> MNNKLMNIIELIRKDTGINNAIDAVEQLALLLLVRYTHEVASNEISKENHIDSFKNLFFDLNDFSKDGLVIDFYTLRDKLNHIVVNCRFSENELSHSVFSRNNWEKIENILDQIPFRIRSTKILDLVIHRLEELDLSEGIEIDFDHLLLNMVKDSGSSGAYYSPRPLIKAMVRVLNPKPLATVYDPAMGTGGVFVEAKKHAKGKSCFNGLSFIGNDLSPFAHLIGALNLLLNDIDISGVSISDSLLDRDCQQYDFVISGVPFGKVNELTKYEY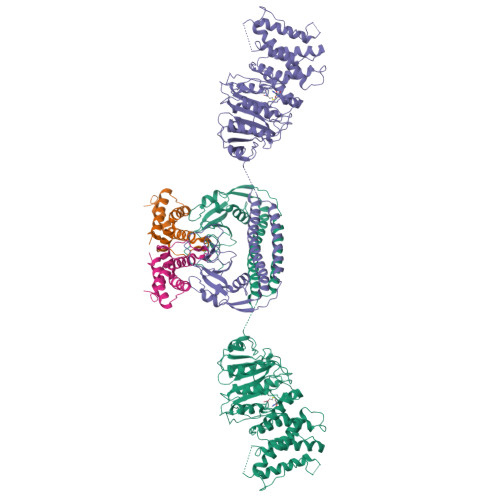YYHGYSGSLEAMFLKHTMDKLAKGGRAAIVIPDGILFGNASHLDELKRQLLTQFNLHAVLSLPKGTLAPYSGVKVSVLFFDNTVSEKDIWFYELRTNKPLSKVNSITDSDFEDFTSLYERREVSENSCLISKESLLQDKTLNLSFSLPKTEAGLKFDKQEMIASLKSEQLSLVTSIENHFDYMSLNLECKYIHQVKLKDICKLRSGDKLNKSEVMDSGEFPVYGGNGVIGFNVEPNRHGDSIVIGKVGAHCGNIHFSTQPYWLTSNAMSLELLDTTKVYLPYLAHVLKSLELNNLATGTAQKFISINKLYEVEVSLPSLEKQREMSEWFTSIEESKSKIQSLLADFSRNLGTISTESITEKALKG;> MAMSNMTYNNVFDHAYEMLKENIRYDDIRDTDDLHDAIHMAADNAVPHYYADIFSVMASEGIDLEFEDSGLMPDTKDVIRILQARIYEQLTIDLWEDAEDLLNEYLEEVEEYEEDEE>MAASTEGVISNKQVILKDYVTGFPKESDMQLTTATTKLKLPEGSKGVLVKNLYLSCDPYMRSRMTKREPGASYVDSFDAGSPIVGYGVAKVLESGDPKFKKGDLIWGMTGWEEYSVITSTESLFKIQHIDVPLSYYTGILGMPGMTAYAGFYEICNPKKGETVFVSAASGAVGQLVGQFAKLLGCYVVGSAGSKEKVDLLKNKFGFDKAFNYKEEPDLDAALKRYFPEGIDIYFENVGGKMLDAVLPNMRVHGRIAVCGLISQYNIDEPEGCRNLMYLIIKQVRMQGFLVFSY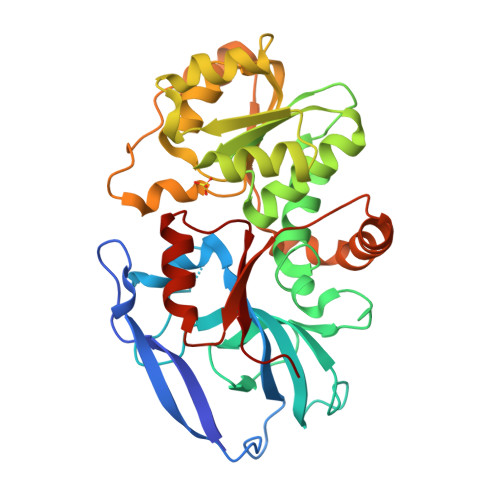YHLYEKFLEMVLPAIKEGKLTYVEDVVEGLESAPAALIGLYAGRNVGKQVVVVSRE[2x]>[2x]GAAALKNYYEVHKELFEGVQKWEETWRLFLEFERKASDPNRFTNRGGNLLKEEKQRAKLQKMLPKLEEELKARIELWEQEHSKAFM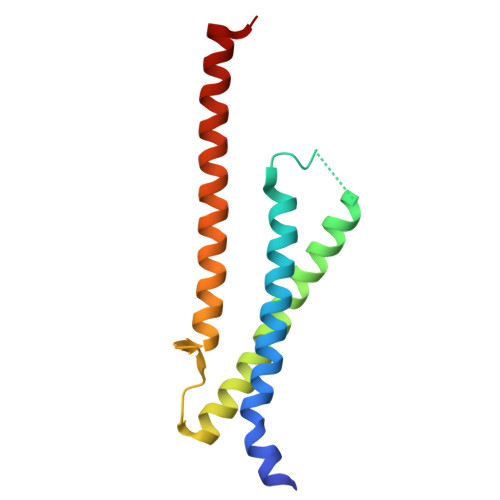VNGQKFMEYVAEQWEMHRLEKERAKQERQLKNKKQTETEMLYGS> CHWLEN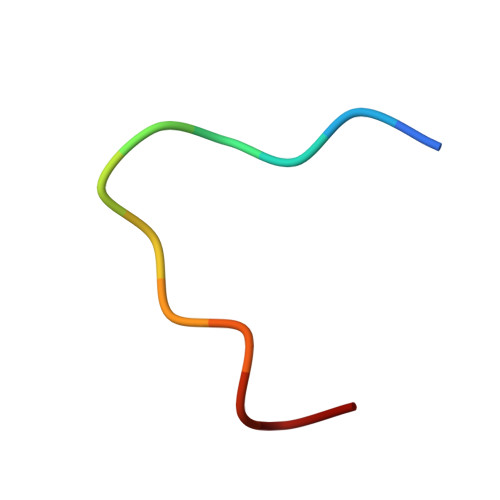CWRGFC>MKRQGKRPSKNLKARCSRKALHVNFKDMGWDDWIIAPLEYEAFHCEGLCEFPLASHL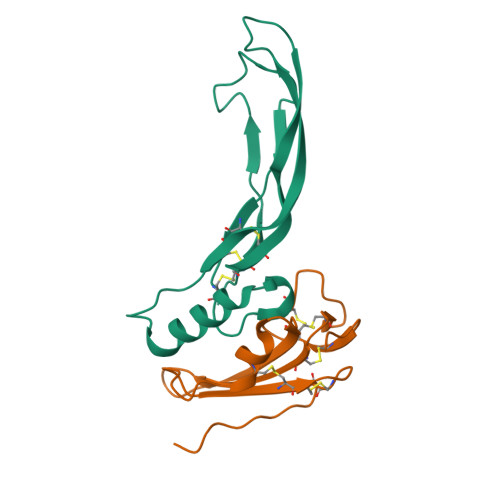EPTNHAVIQTLMNSMDPESTPPTCCVPTRLSPISILFIDSANNVVYKQYEDMVVESCGCR[2x];>[2x]GSGAMAQNLDSMLHGTGMKSDSDQKKSENGVTLAPEDTLPFLKCYCSGHCPDDAINNTCITNGHCFAIIEEDDQGETTLASGCMKYEGSDFQCKDSPKAQLRRTIECCRTNLCNQYLQPTLPPVVIGPFFDGSIR(1R,2R,3S,4R,6S)-4,6-diamino-2-{[3-O-(2,6-diamino-2,6-dideoxy-beta-L-idopyranosyl)-2-O-{2-[(2-phenylethyl)amino]ethyl}-beta-D-ribofuranosyl]oxy}-3-hydroxycyclohexyl 2-amino-2-deoxy-alpha-D-glucopyranoside | C33 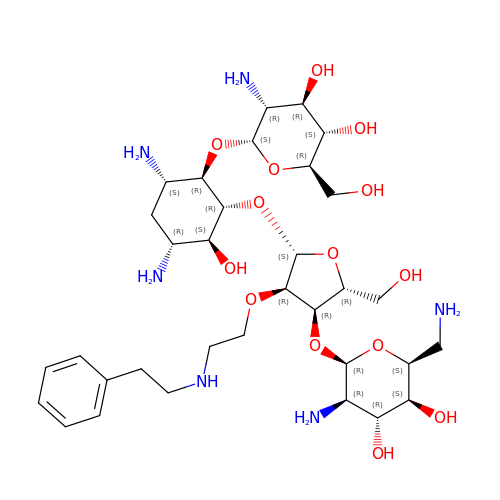H58 N6 O14 | RYWOYAQAVIFICV-KWRLVFCDSA-N Here we report near-atomic models built into cryo-EM structures of procapsid I, intermediate procapsid II which has partially released the SP, and the mature DNA-filled capsid from bacteriophage SPP1. The structures are T = 7 laevo icosahedra composed of 415 copies of the MCP gp13 (35.4 kDa), several hundred copies of SP gp11 (23.5 kDa) inside procapsids, 180 copies of gp12 in DNA-filled capsids, and a gp6-gp7 complex which forms the specialised portal vertex. The asymmetric units (ASUs) comprise seven SPP1 gp13 subunits: six in a hexon (subunits A to F) and one from the capsid penton (subunit G). Gp13 has the characteristic L-shape of capsid proteins of other tailed bacteriophages, with well-defined A and P domains, an extended N-terminus arm, and the E-loop.

Procapsid II is larger, more angular and has a much thinner shell than procapsid I, ranging between 2 and 2.7 nm. Procapsid II has bulky density for the SP attached to the capsid lattice interior only underneath the MCP five−fold vertices. The hexon becomes less skewed in procapsid II, more flat and expands to a size of 16.5 nm × 14.2 nm with the central opening getting slightly larger (~3.0 nm × 3.7 nm). The transition from procapsid I to procapsid II is induced by major structural rearrangements in the hexon subunits that become flattened resulting in expansion without major changes in the pentons. Subunits A-E of the ASU undergo significant conformational changes in the P domains and N-arms during transition from procapsid I to procapsid II. In procapsid I all MCP subunits are bound to the SP gp11 protein via the N-terminal helix α1* (Phe15-Leu26), positioned beneath the capsid shell and the N-terminus of the spine helix α3 from the same subunit. These interactions are disrupted in subunits A–E of procapsid II where helices α1* unfold to an extended strand similar to the one found in the MVC. The N-terminus arm moves upwards by 60° and stretches out from the P domain towards the hexon periphery, protruding to the outer surface. The A and P domains of subunits F and G keep a similar conformation in the two procapsid states, correlating with maintenance of their attachment to the SP, while the E-loop moves outwards making the overall conformation more flat. In the SPP1 procapsid II intermediate state, SPs are associated only to MCP subunit F of hexons and to all subunits forming pentons (central panel), demonstrating that this interaction is more stable than the one of SP bound exclusively to hexons. Each N-arm of the MCP Ci subunit forms four contacts with the MCP D(i + 1) subunit from the neighbouring ASU in procapsid II.

>AYTKISDVIVPELFNPYVINTTTQLSAFFQSGIAATDDELNALAKKAGGGSTLNMPYWNDLDGDSQVLNDTDDLVPQKINAGQDKAVLILRGNAWSSHDLAATLSGSDPMQAIGSRVAAYWAREMQKIVFAELAGVFSNDDMKDNKLDISGTADGIYSAETFVDASYKLGDHESLLTAIGMHSATMASAVKQDLIEFVKDSQSGIRFPTYMNKRVIVDDSMPVETLEDGTKVFTSYLFGAGALGYAEGQPEVPTETARNALGSQDILINRKHFVLHPRGVKFTENAMAGTTPTDEELANGANWQRVYDPKKIRIVQFKHRLQA[7x]> MANMKNSNDRIILFRKAGEKVDATKMLFLTEYGLSHEADTDTEDTMDGSYNTGGSVESTMSGTAKMFYGDDFADEIEDAVVDRVLYEAWEVESRIPGKNGDSAKFKAKYFQGFHNKFELKAEANGIDEYEYEYGVNGRFQRGFATLPEAVTKKLKATGYRFHDT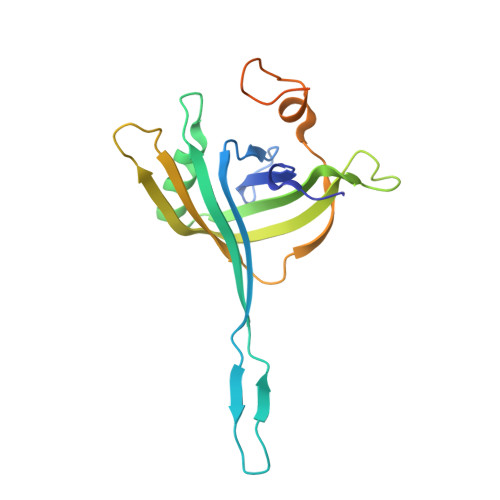TKEDALTSEDLTAIPQPKVDSSTVTPGEV>TIKVGINGFGRIGRIVFRAAQKRSDIEIVAINDLLDADYMAYMLKYDSTHGRFDGTVEVKDGHLIVNGKKIRVTAERDPANLKWDEVGVDVVAEATGLFLTDETARKHITAGAKKVVMTGPSKDNTPMFVKGANFDKYAGQDIVSNASCTTNCLAPLAKVINDNFGIIEGLMTTVHATTATQKTVDGPSHKDWRGGRGASQNIIPSSTGAAKAVGKVLPELNGKLTGMAFRVPTPNVSVVDLTVRLEKAATYEQIKAAVKAAAEGEMK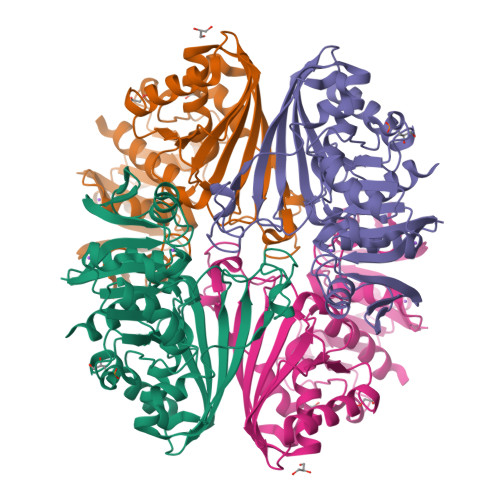GVLGYTEDDVVSTDFNGEVCTSVFDAKAGIALNDNFVKLVSWYDNETGYSNKVLDLIAHISK[2x]>[3x]HHHHHHLVPRGSMSNKLITDLSRVFDYRYVDENEYNFKLISDMLTDFNFSLEYHRNKEVFAHDGEQIKYEHLNVTSNVSDFLTYLNGRFSNMVLGHNGDGINEVKDARVDNTGYGHKTLQDRLYHDYSTLDVFTKKVEKAVDEHYKEYRATEYRFEPKEQEPEFITDLSPYTNAVMQSFWVDPRTKIIYMTQARPGNHYMLSRLKPNGQFIDRLLVKNGGHGTHNAYRYIDGELWIYSAVLDSNKNNKFVRFQYRTGEITYGNEMQDVMPNIFNDRYTSAIYNPVENLMIFRREYKPTERQLKNSLNFVEVRSADDIDKGIDKVLYQMDIPMEYTSDTQPMQGITYDAGILYWYTGDSNTANPNYLQGFDIKTKELLFKRRIDIGGVNNNFKGDFQEAEGLDMYYDLETGRKALLIGVTIGPGNNRHHSIYSIGQRGVNQFLKNIAPQVSMTDSGGRVKPLPIQNPAYLSDITEVGHYYIYTQDTQNALDFPLPKAFRDAGWFLDVLPGHYNGALRQVLTRNSTGRNMLKFERVIDIFNKKNNGAWNFCPQNAGYWEHIPKSITKLSDLKIVGLDFYITTEESNRFTDFPKDFKGIAGWILEVKSNTPGNTTQVLRRNNFPSAHQFLVRNFGTGGVGKWSLFEGKVVE

Gp45 of ϕ11 was identified and characterized as the receptor-binding protein (RBP) of ϕ11 9. Furthermore, it was shown that ϕ11 was unable to bind to the cell wall in the absence of WTA–GlcNAc, identifying glycosylated WTA as the receptor. Although phages are the most abundant and diversified biological entity on earth, each phage can only infect a limited number of bacterial strains. This specific phage-host interaction is determined, in part, by the protein recognition device located at the tip of the phage tail, which engages a receptor at the bacterial cell surface. The RBP structure reveals a trimer with a complex fold that can be divided, from N- to C-terminus, into a “stem”, a “platform” and a “tower”.

The RBP of ϕ11 assembles into an elongated homotrimer, with overall dimensions of approximately 160 × 120 × 100 Å. The stem is formed by a long, severely bent triple α-helical coiled coil that features three interruptions: the first and third interruptions are both β-hairpin structures and the second is a short disordered region. A strong electron density feature suggesting the presence of a metal ion was observed at the junction between the first two bundles. Using an RBP crystal and extended X-ray absorption fine structure (EXAFS) spectroscopy, the identity of this ion was determined to be iron, which probably exists in its oxidized form Fe3+ (analyzed at SOLEIL beamline PX1). The Fe3+ ion is positioned along the 3-fold axis of the first helix bundle and coordinated by the side chains of His42 and His50 from each of the three monomers. We therefore suggest that it serves a different role, perhaps by helping to stabilize the bundles that undergo a sharp turn at the hinge. While the first and second helical bundles are collinear, the hinge introduces a sharp angle of ~30° between the second and the third bundle. Helix α3 (residues 88–97), a short triple helical coil located in the hinge, has an independent rotation axis not aligned to the remainders of the molecule. This helical bundle is followed by five-bladed β-propeller modules of the platform, which encompass residues 142–439 and form the midsection of the protein. Contacts between the three propeller domains are sparse, as each interface between two propeller domains buries a surface area of only 457 Å2 from solvent, and much of this surface is buried due to a helix-helix contact at the center of the trimer axis. The cavity is lined with polar residues (Gln165, Thr211, Gln330), which could serve to establish hydrogen bonds with the modelled GlcNAc molecule.> AAQTNAPWGLARISSTSPGTSTYYYDESAGQGSCVYVIDTGIEASHPEFEGRAQMVKTYYYSSRDGNGHGTHCAGTVGSRTYGVAKKTQLFGVKVLDDNGSGQYSTIIAGMDFVASDKNNRNCPKGVVASLSLGGGYSSSVNSAAARLQSSGVMVAVAAGNNNADARNYSPASEP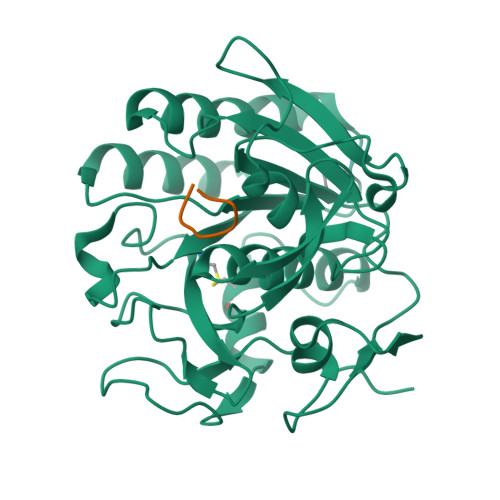SVCTVGASDRYDRRSSFSNYGSVLDIFGPGTSILSTWIGGSTRSISGTSMATPHVAGLAAYLMTLGKTTAASACRYIADTANKGDLSNIPFGTVNLLAYNNYQA;> GDEQGENK1,2-DI-N-PENTANOYL-SN-GLYCERO-3-DITHIOPHOSPHOCHOLINE | C18 H36 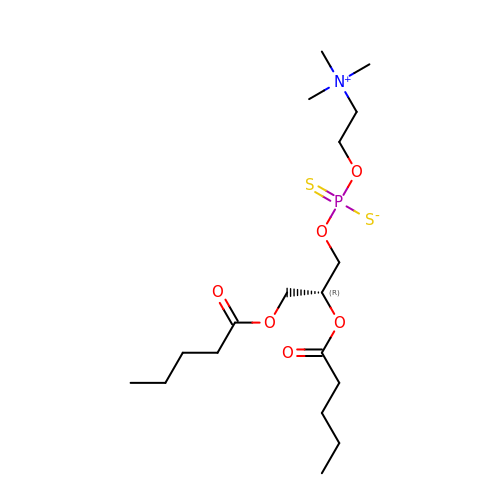N O6 P S2 | WEXRBKRFCBLWEL-MRXNPFEDSA-N>[2x]SDKQKAINYLMQFAHKVSGKYRGVAKLEGNTKAKVLQVLATFAYADYCR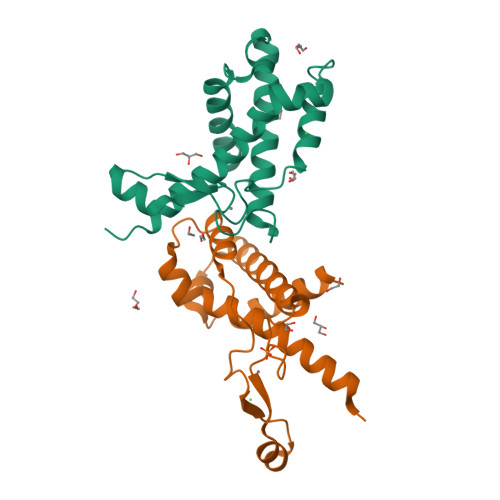SAATPGARCRDCHGTGRAVDIAKTKLWGRVVEKECGRCKGVGYSRMPASAAYRAVTMLIPNLTQPTWSRTVKPLYDALVVQCHKEESIADNILNAVTR>MRSRRVDVMDVMNRLILAMDLMNRDDALRVTGEVREYIDTVKIGYPLVLSEGMDIIAEFRKRFGCRIIADFKVADIPETNEKICRATFKAGADAISVHGFPGADSVRACLNVAEEMGREVFLLTEMSHPGAEMFIQGAADEIARMGVDLGVKNYVGPSTRPERLSRLREIIGQDSFLISPGVGAQGGDPGETLRFADAIIVGRSIYLADNPAAAAAGIIESIKDLLNP[2x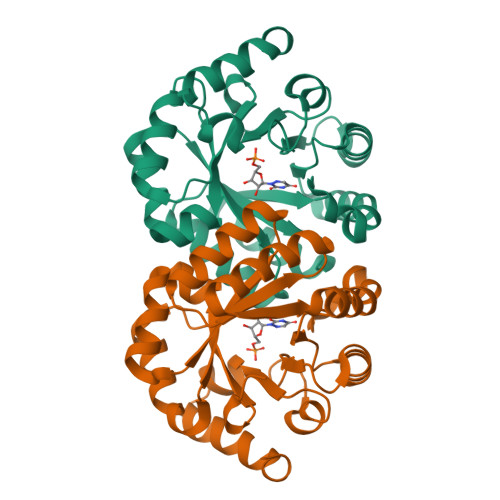]>[3x]CGCTAT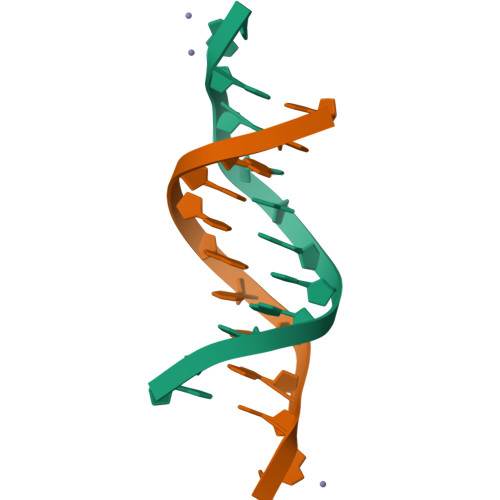AATGCG;>[3x]GGCATTATAGCG Isocitrate dehydrogenase (IDH) catalyzes the oxidative decarboxylation of isocitrate to produce α-ketoglutarate and CO2 while reducing the cofactor nicotinamide adenine dinucleotide (phosphate) (NAD(P)+) to NAD(P)H using divalent metal cation (Mg2+ or Mn2+) in the tricarboxylic acid cycle. Although the amino acid sequence identity between subfamilies I and II is low (<20%), both IDHs function as homodimers; each monomer is composed of three domains: large, small, and clasp domains, and the active site is situated between the large and small domains. The thermoacidophilic archaeon Sulfolobus tokodaii strain 7, which grows optimally at 75°C and pH 3, has an open reading frame ST2166 in the genome encoding hypothetical IDH. In this study, we expressed, purified, and determined the crystal structures of ST2166 in the apo and NADP+-bound forms at 2.0 Å and 2.4 Å resolutions, respectively, and discussed the mechanisms for cofactor recognition of prokaryotic NADP-IDHs.

ST2166 crystallized in a monoclinic crystal belonging to P21 that diffracted X-rays up to 2.0 Å resolution. In this crystal, the asymmetric unit contains two monomers having nearly identical overall structures with root-mean-square deviation (RMSD) for least-squares fitting of Cα atoms of 0.18 Å. The final model comprises 401 amino acid residues per subunit and 463 water molecules. Residues 101–108, part of the Cd loop and d helix (residues 97–118) equivalent to the phosphorylation loop in EcIDH, are disordered. Each subunit containing 17 α-helices and 15 β-strands is subdivided into the large domain (residues 1–120 and 302–409), the small domain (residues 121–153 and 196–301), and the clasp domain (residues 154–195). In the structure of the apo form, putative isocitrate-binding residues (Ser109, Asn111, Arg115, Arg125, Arg149, Asp298, Tyr156, Lys223′, Asn225′, and Arg274′, the prime designates a residue from the adjacent subunit) involved in the binding of isocitrate in prokaryotic NADP-IDHs are exposed to the inner surface in the deep cleft of the active site. Therefore, it is probable that ST2166 has the same catalytic mechanism as proposed for other prokaryotic NADP-IDHs. The apo crystal of ST2166 was easily cracked upon soaking with citrate but not NADP+, suggesting that citrate mimicking the substrate isocitrate can bind to the opening active site of the enzyme and induce a large conformational change to break the crystal lattice. Therefore, binding of NADP+ is not necessary for a large domain movement in ST2166.

>[2x]MLYKEPEDGEKIKFDKGKWIVPNKPVILYIEGDGIGPEITNAAIKVINKAVERAYGSSREIKWLEVYAGEKAEKLVNDRFPKETQEMLLKYRVVLKGPLETPIGKGWKSVNVAIRLMLDLYANIRPVKYIEGLESPLKHPEKVDMIIFRENTDDLYRGIEYPFNSEEAKKIRDFLRKELKVEIEDDTGIGIKVMSKYKTQRITRLAIQYAIEHKRKKVTIMHKGNVMKYTEGAFREWAYEVALKEYRDFIVTEEEINQGKPDQGKIILNDRIADNMFQQIIIRPEEYDIILAPNVNGDYISDAAGALIGNIGMLGGANIGDEGGMFEAIHGTAPKYAGKNVANPTGIIKAGELMLRWMGWNEAADLIEKAINMAIRDKKVTQDIARFMGVKALGTKEYADELIKIMDTI>AAGVAAWLPFARAAAIGWMPVASGPMPAPPRQERKRTQDALIVLNVSGTRFQTWQDTLERYPDTLLGSSERDFFYHPETQQYFFDRDPDIFRHILNFYRTGKLHYPRHECISAYDEELAFFGLIPEIIGDCCYEEYKDRRRENAERLQDDADTDTAGESALPTMTARQRVWRAFENPHTSTMALVFYYVTGFFIAVSVIANVVETVPCGSSPGHIKELPCGERYAVAFFCLDTACVMIFTVEYLLRLAAAPSRYRFVRSVMSIIDVVAILPYYIGLVMTDNEDVSGAFVTLRVFRVFRIFKFSRHSQGLRILGYTLKSCASELGFLLFSLTMAIIIFATVMFYAEKGSSASKFTSIPAAFWYTIVTMTTLGYGDMVPKTIAGKIFGSICSLSGVLVIALPVPVIVSNFSRIYHQNQRADKRRAQKKARLARIRAAKSGSANAYMQSKRSGLLSNQGRGDGSAFVTKSGSSFETQHHHLLHCLEKTTNHEFVD[4x];>PEGLEQLEAQTNFTKRELQVLYRGFKNECPSGVVNEDTFKQIYAQFFPHGDASTYAHYLFNAFDTTQTGSVKFEDFVTALSILLRGTVHEKLRWTFNLYDINKDGYINKEEMMDIVKAIYDMMGKYTYPVLKEDTPRQHVDVFFQKMDKNKDGIVTLDEFLESCQEDDNIMRSLQLFQNVM[4x]

Modulation of voltage-gated potassium (Kv) channels by auxiliary subunits is central to the physiological function of channels in the brain and heart. Native Kv4 tetrameric channels form macromolecular ternary complexes with two auxiliary β-subunits—intracellular Kv channel-interacting proteins (KChIPs) and transmembrane dipeptidyl peptidase-related proteins (DPPs)—to evoke rapidly activating and inactivating A-type currents, which prevent the backpropagation of action potentials. Here we report cryo-electron microscopy structures of the Kv4.2–DPP6S–KChIP1 dodecamer complex, the Kv4.2–KChIP1 and Kv4.2–DPP6S octamer complexes, and Kv4.2 alone. Thus, our data suggest that two distinct modes of modulation contribute in an additive manner to evoke A-type currents from the native Kv4 macromolecular complex.

The structures of Kv4.2–KChIP1 show that the Kv4.2 protomer comprises an N-terminal cytoplasmic domain with an N-terminal hydrophobic segment of approximately 40 residues in length (referred to as the inactivation ball), the T1 domain, a transmembrane domain with six transmembrane helices S1–S6, and the C-terminal cytoplasmic domain. The C-terminal intracellular S6 helix continuously extends from the transmembrane S6 helix toward KChIP1, which was not observed in previous studies. In addition, the intracellular S6 helix interacts with the T1–S1 linker in the structure of the Kv4.2–KChIP1 complex. The Kv4-specific topology of the T1 domain would facilitate the proper interaction between the intracellular S6 helix and KChIP1. The present structure of the full-length Kv4.2–KChIP1 complex reveals that the C terminus of Kv4.2 tightly interacts with both KChIP1 and the N terminus of Kv4.2. The C-terminal cytoplasmic S6 helix continuously extends from the transmembrane S6 helix and terminates at S450, which is localized at the bottom of the complex. The structural comparison between Kv4.2 alone and the Kv4.2–KChIP1 complex provides insight into how KChIPs modulate the gating of Kv4s. First, one KChIP1 stabilizes the S6 conformation as well as the N terminus from the neighbouring subunit of Kv4.2. Third, previous functional studies have suggested that the T1–S1 linker of Kv4 dodecameric channels undergoes major conformational shifts tightly coupled to movements of the S6 tail, although we do not know what the T1 conformational change is. Together, these structural features mediated by KChIP1 may allow synchronized and accelerated S6 gating to enable fast CSI and recovery.>PGEDRFKPVVPWPHVEGVEVDLESIRRINKAKNEQEHHAGGDSQKDIMQRQYLTFKPQTFTYHDPVLRPGILGNFEPKEPEPPGVVGGPGEKAKPLVLGPEFKQAIQASIKEFGFNMVASDMISLDRSVNDLRQEECKYWHYDENLLTSSVVIVFHNE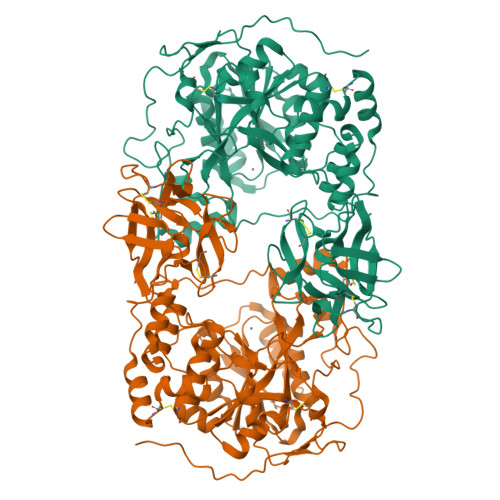GWSTLMRTVHSVIKRTPRKYLAEIVLIDDFSNKEHLKEKLDEYIKLWNGLVKVFRNERREGLIQARSIGAQKAKLGQVLIYLDAHCEVAVNWYAPLVAPISKDRTICTVPLIDVINGNTYEIIPQGGGDEDGYARGAWDWSMLWKRVPLTPQEKRLRKTKTEPYRSPAMAGGLFAIEREFFFELGLYDPGLQIWGGENFEISYKIWQCGGKLLFVPCSRVGHIYRLEGWQGNPPPIYVGSSPTLKNYVRVVEVWWDEYKDYFYASRPESQALPYGDISELKKFREDHNCKSFKWFMEEIAYDITSHYPLPPKNVDWGEIRGFETAYCIDSMGKTNGGFVELGPCHRMGGNQLFRINEANQLMQYDQCLTKGADGSKVMITHCNLNEFKEWQYFKNLHRFTHIPSGKCLDRSEVLHQVFISNCDSSKTTQKWEMNNIHSV[6x]> MVILKVAEWGGRPAKRMLDAQQLPINRVVISHTAAEGCESREVCSARVNVVQSFHMDSWGWDHIGYNFLVGGDGRVYEGRGWDYVGAHTKGYNRGSIGISFIGTFTTRKPNERQLEACQLLLQEGVRLKKLTTNYRLYGHRQLSATESP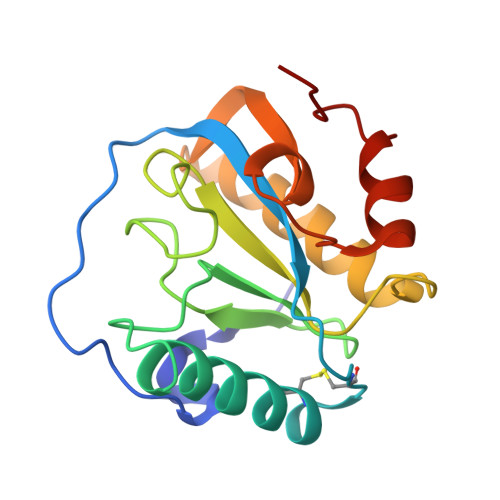GEELYKIIKKWPHWSHEI> MERYENLFAQLNDRREGAFVPFVTLGDPGIEQSLKIIDTLIDAGADALELGVPFSDPLADGPTIQNANLRAFAAGVTPAQCFEMLAIIREKHPTIPIGLLMYANLVFNNGIDAFYARCEQVGVDSVLVADVPVEESAPFRQAALRHNIAPIFICPPNADDDLLRQVASYGRGYTYLLSRSGVVGAENRGALPLHHLIEKLKEYHAAPALQGFGISSPEQVSAAVRAGAAGAISGSAIVKIIEKNLASPKQMLAELRSFVSAMKAASRA;> MTTLLNPYFGEFGGMYVPQILMPALNQLEEAFVSAQKDPEFQAQFADLLKNYAGRPTALTKCQNITAGTRTTLYLKREDLLHGGAHKTNQVLGQALLAKRMGKSEIIAETGAGQHGVASALASALLGLKCRIYMGAKDVERQSPNVFRMRLMGAEVIPVHSGSATLKDACNEALRDWSGSYETAHYMLGTAAGPHPYPTIVREFQRMIGEETKAQI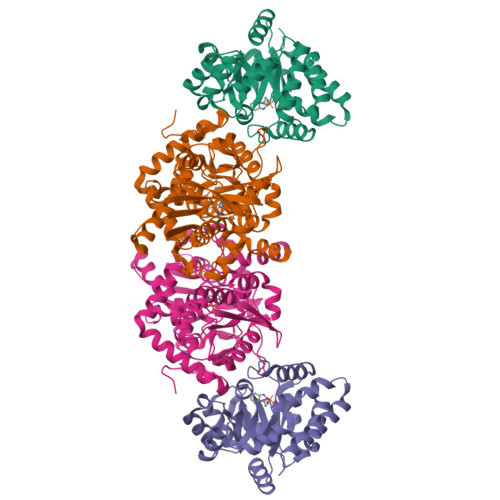LDKEGRLPDAVIACVGGGSNAIGMFADFINDTSVGLIGVEPGGHGIETGEHGAPLKHGRVGIYFGMKAPMMQTADGQIEESYSISAGLDFPSVGPQHAYLNSIGRADYVSITDDEALEAFKTLCRHEGIIPALESSHALAHALKMMREQPEKEQLLVVNLSGRGDKDIFTVHDILKARGEI>SNAMIRKYRYGAPFDTEALTEKIETAEEAFPYGEISQKEGFAFTYIMDEDDIVYGLGESNRGINKRGYCYISNCTDDPIHTEDKRSLYGAHNFIIVSGKTTFGLFFDYPSKLTFDIGYTRMDTLKVSCENADLDIYVIEGENAYDIVKQFRRVIGRSYIPPKFAFGFGQSRYGYTTKEDFRAVAKGYRENHIPIDMIYMDIDYMQDFKDFTVNEKNFPDFPEFVKEMKDQELRLIPIIDAGVKVEKGYEVYEEGVKNNYFCKREDGSDFVAAVWPGDTHFPDMLNPEARKWFGDKYRFLIDQGIEGFWNDMNEPAIFYSSEGLAEAKEFAGEFAKDTEGKIHPWAMQAKMKDIVNSPEDYKRFYHNVNGKKIRHDKVHNLFGYNMTRAAGEAFERIDPEKRFLMFSRSSYIGMHRYGGIWMGDNKSWWSHILLNLKMLPSLNMCGFMYTGADLGGFGDDTTRDLLLRFLALGVFTPLMRDHAAEGTREQECYQFENIEDFRSVINARYRLVPYLYSEYMKAALNDDMYFKPLGFVYPDDKMAIRVEDQLMLGNEIMIAPVYEQNARGRYVYLPEEMKFIKFMPDGSISEEVLEKGVHYVDVALNEVPL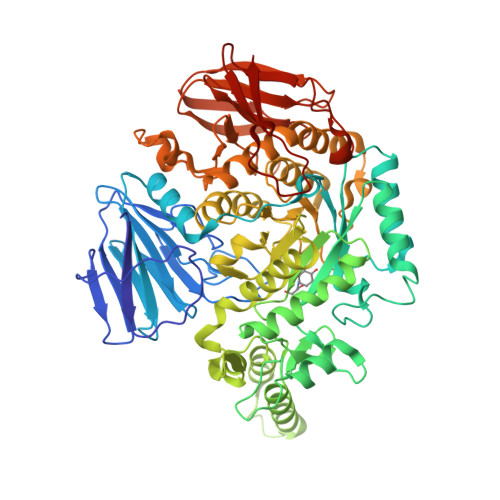FIRSGKCIPVAEAAECVKDIDTENMQLIGYEGSSYTLYEDDGIHKDYDKKENYRVLTK[2x]>MKKSELPDPFEKARESKGYGEMNDQDDPVTMLLRHKDVRKSAHNYKTFQSGAVPGRIVIPSEVDIRDTRQIPFEVDPPVHGVYRAIVEPWFKRP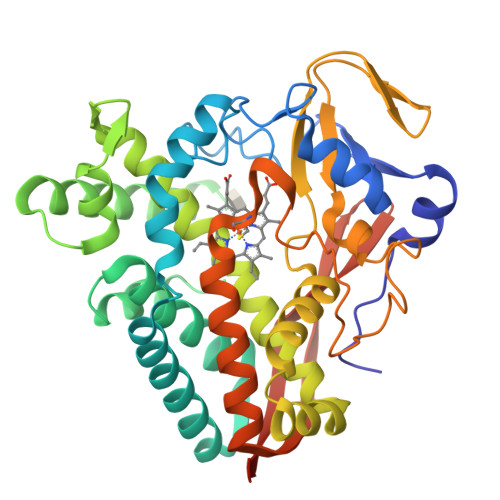LQAEYQEKLTAQISEIVEETLLKGSVEVVTDFALRLQSRALTLLLNTPFSESETWISWGTHVFRSEGEALDGDKANILYHYIDEQIDRASENPGDDMYSVLLNSEFEGRKLTKEEVKGVMVLTFAGGRDTVINAVTNSIAYLAEHPEALERLRKEPEITGRAVEEMIRYFSPLTQMGRVVTEDTHVCEHAVKADSRISLCWASANRDAAVFENPNEIVLDRKVNPHVGFGFSHHNCLGATHARQILKILLQTLAQKVASFEILDYKENIEDLDHFQRKVGFHNIQIKFNPLTKLAAALEHHHHHH[2x]> MKSSGAHGNVMGDAGVLKNEDESKYLDQVRYILKNGERIDDRTGVGTISVFGMHSVYSLRNGVVPVLTTKRVYWKGVVEELLWFIRGDTNAKHLSEKGVRIWDANGSRQFLDQCGFSDRSEGDLGPIYGFQWRHCGAEYRGMDTDYTNQGIDQLSEIIDLIKNEPHSRRIILSAWNVKDLKLMALPPCHTLAQFAVRNGELSCQLYQRSGDMGLGVPFNLASYGLLTHMIAHVCG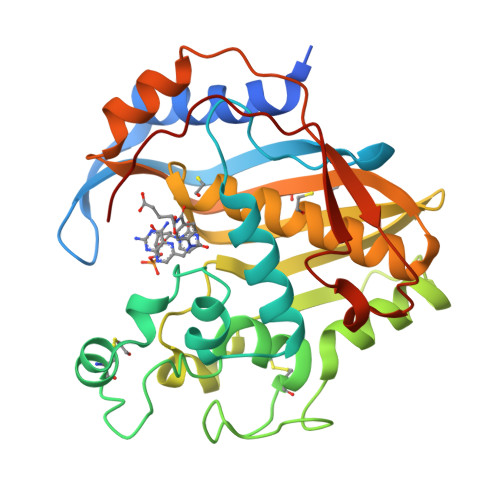LKTGHLCHVLGDAHVYMNHVDALQEQLKRQPRQFPTVRFIGNIKTIDDFTYESIVLENYQPMPAIKMAMAV N-{2-[(5-chloro-2-{[4-(4-methylpiperazin-1-yl)phenyl]amino}pyrimidin-4-yl)oxy]phenyl}prop-2-enamide 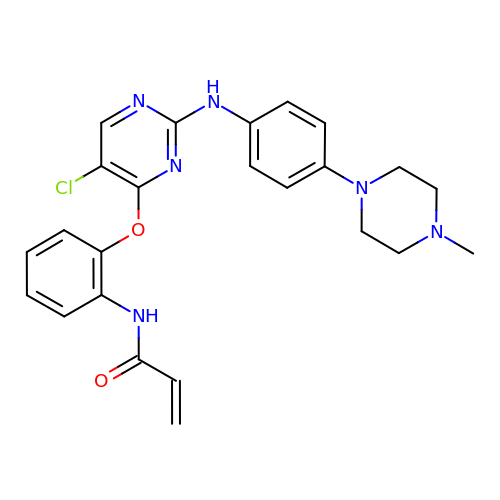| C24 H25 Cl N6 O2 | WOQNVLPDIGPVKR-UHFFFAOYSA-N The gp43 DNA polymerase of the RB69 bacteriophage (RB69 Pol) bears primary responsibility for the faithful and efficient replication of the viral genome. RB69 Pol belongs to the B-class of DNA polymerases and is closely related to T4 phage DNA polymerase. RB69 DNA Pol synthetizes DNA with high accuracy, introducing one mutation per 2 x 108 replicated bases. This high fidelity is achieved through the combined action of its polymerase (Pol) and 3′-5′-exonuclease (Exo) activities, which enable stringent selection of the correct incoming nucleotide and excision of the mismatches resulting from misincorporations.

In order to understand the mechanism underlying this effect at the atomic level, we first crystallized and solved the structure of the PolD714A apoenzyme at 2.60 Å resolution. Detailed analysis of the region surrounding the D714 residue reveals, however, an interesting rearrangement of a hydrogen bond network propagating from the site of the substitution towards the catalytic center of the polymerase. Inspection of the omit map calculated for the 712-724 residues of PolD714A structure, at a contour level as low as 1.5σ, confirms the presence of the D714A substitution, as well as the appearance of structural distortions in the vicinity of the replaced residue. These changes are most probably the immediate consequence of the abrogation of polar D714 side chain interactions. The new conformation of E716 appears to be stabilized by a 2.7 Å hydrogen bond between the O-ε atoms of E716 and E686. The movement of E716 most likely triggers a shift of its surrounding residues, in particular R719, Y720, E722 and K724, which comprise the 27-28 β-sheets surface of the RB69 Pol palm subdomain. Importantly, the distortions of the hydrogen bond network around the A714 amino acid domino out towards the polymerizing center of the enzyme and eventually affect the position of the catalytically essential D411. The D411 residue, located approximately 15 Å away from D714, displays a large rotation of the side chain and a slight 0.3 Å shift of the C-α atom. These rearrangements are most likely a consequence of the new conformation of E686, as both residues are spatially close in the native apoenzyme structure.

> MKEFYLTVEQIGDSIFERYIDSNGRERTREVEYKPSLFAHCPESQATKYFDIYGKPCTRKLFANMRDASQWIKRMEDIGLEALGMDDFKLAYLSDTYNYEIKYDHTKIRVANFDIEVTSPDGFPEPSQAKHPIDAITHYDSIDDRFYVFDLLNSPYGNVEEWSIEIAAKLQEQGGDEVPSEIIDKIIYMPFDNEKELLMEYLNFWQQKTPVILTGWNVESFAIPYVYNRIKNIFGESTAKRLSPHRKTRVKVIENMYGSREIITLFGISVLDYIDLYKKFSFTNQPSYSLDYISEFELNVGKLKYDGPISKLRESNHQRYISYNIIAVYRVLQIDAKRQFINLSLDMGYYAKIQIQSVFSPIKTWDAIIFNSLKEQNKVIPQGRSHPVQPYPGAFVKEPIPNRYKYVMSFDLTSLYPSIIRQVNISPETIAGTFKVAPLHDYINAVAERPSDVYSCSPNGMMYYKDRDGVVPTEITKVFNQRKEHKGYMLAAQRNGEIIKEALHNPNLSVDEPLDVDYRFDFSDEIKEKIKKLSAKSLNEMLFRAQRTEVAGMTAQINRKLLINSLYGALGNVWFRYYDLRNATAITTFGQMALQWIERKVNEYLNEVCGTEGEAFVLYGDTDSIYVSADKIIDKVGESKFRDTNHWVDFLDKFARERMEPAIDRGFREMCEYMNNKQHLMFMDREAIAGPPLGSKGIGGFWTGKKRYALNVWAMEGTRYAEPKLKIMGLETQKSSTPKAVQKALKECIRRMLQEGEESLQEYFKEFEKEFRQLNYISIASVSSANNIAKYDVGGFPGPKCPFHIRGILTYNRAIKGNIDAPQVVEGEKVYVLPLREGNPFGDKCIAWPSGTEITDLIKDDVLHWMDYTVLLEKTFIKPLEGFTSAAKLDYEKKASLFDMFDF>GSHMSNTQTVLPFTGLNTPSGVAVDSAGTVWVTDHGNNRVVKLAAGSNTQTVLPFTGLNTPSGVAVDSAG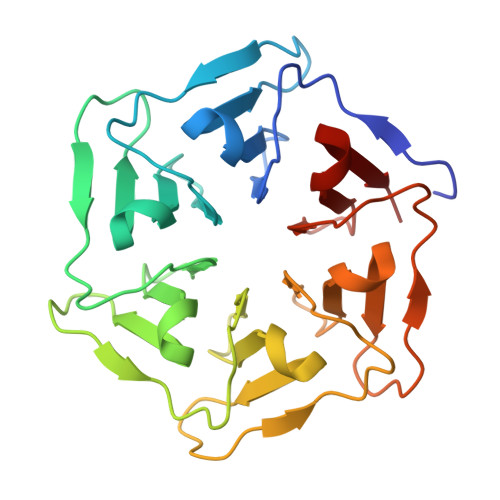TVWVTDHGNNRVVKLAAGSNTQTVLPFTGLNTPSGVAVDSAGTVWVTDHGNNRVVKLAAGSNTQTVLPFTGLNTPSGVAVDSAGTVWVTDHGNNRVVKLAAGSNTQTVLPFTGLNTPSGVAVDSAGTVWVTDHGNNRVVKLAAGSNTQTVLPFTGLNTPSGVAVDSAGTVWVTDHGNNRVVKLAAG[2x]> SDE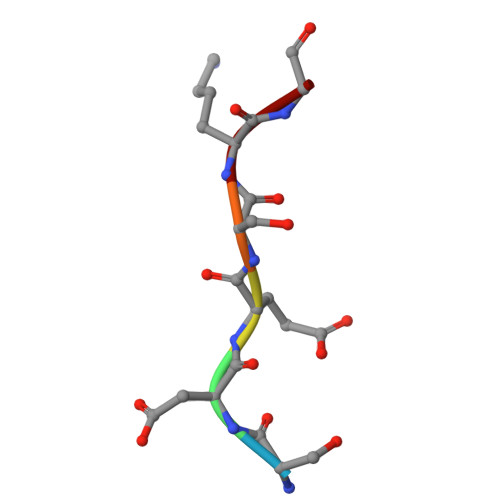SKG> GPLGSMQQKQVNVIEFFSGIGGLRSSYERSSININATFIPFDINEIANKIYSKNFKEEVQVKNLDSISIKQIESLNCNTWFMSPPCQPYNNSIMSKHKDINDPRAKSVLHLYRDILPYLINKPKHIFIENVPLFKESLVFKEIYNILIKNQYYIKDIICSPIDIGIPNSRTRYYVMARLTPFKNEIQLHQEKESMISNYL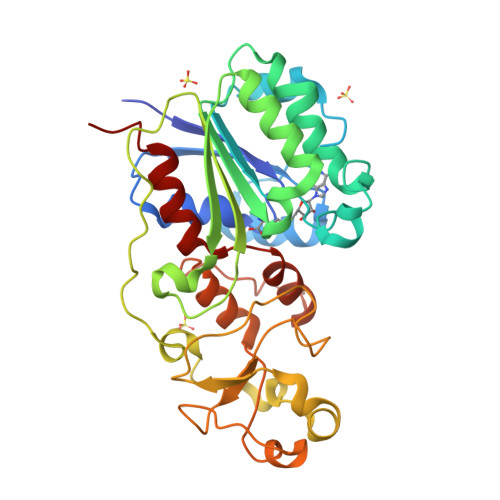DNNVNESYSIPSDLILKKGMLFDIVGKDDKRTCCFTKSYTKIVEGTGSIYCPIEPHFIPVKKAEDLLNKNLRYFTPNEIKKIHGFSSNFTTQIDGLTDKQQYQCLGNSVSCFVIAQLMEYLFDDLKE> DNENVVNEYSSELEKHQLYIDETVNSNIPTNLRVLRSILENLRSKIQKLESDVSAQMEYCRTPCTVSCNIPVVSGKECEEIIRKGGETSEMYLIQPDSSVKPYRVYCDMNTENGGWTVIQNRQDGSVDFGRKWDPYKQGFGNVATNTDGKNYCGLPGEYWLGNDKISQLTRMGPTELLIEMEDWKGDKVKAHYGGFTVQNE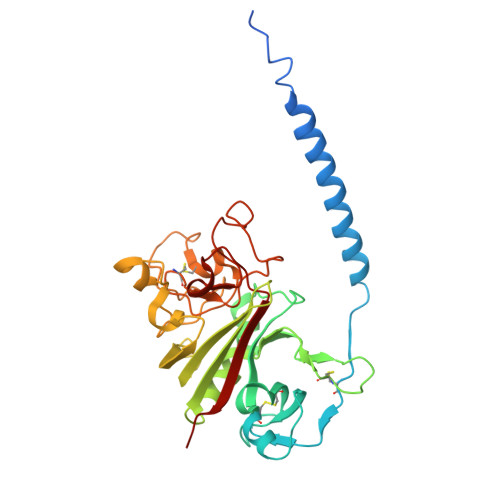ANKYQISVNKYRGTAGNALMDGASQLMGENRTMTIHNGMFFSTYDRDNDGWLTSDPRKQCSKEDGGGWWYNRCHAANPNGRYYWGGQYTWDMAKHGTDDGVVWMNWKGSWYSMRKMSMKIRPFFP>MGGSHHHHHHRSESTVTEELKEGIDAVYPSLVGTADSKAEGIKNYFKLSFTLPEEQKSRTVGSEAPLKDVAQALSSRARYELFTEKETANPAFNGEVIKRYKELMEHGEGIADILRSRLAKFLNTKDVGKRFAQGTEANRWVGGKLLNIVEQDGDTFKYNEQLLQTAVLAGLQWRLTATSNTAIKDAKDVAAITGIDQALLPEGLVEQFDTGMTLTEAVSSLAQKIESYWGLSRNPNAPLGYTKGIPTAMAAEILAAFVESTDVVENIVDMSEIDPDNKKTIGLYTITELDSFDPINSFPTAIEEAVLVNPTEKMFFGDDIPPVANTQLRNPAVRNTPEQKAALKAEQATEFYVHTPMVQFYETLGKDRILELMGAGTL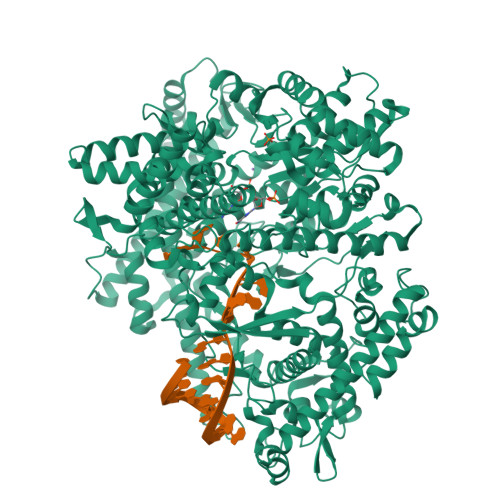NKELLNDNHAKSLEGKNRSVEDSYNQLFSVIEQVRAQSEDISTVPIHYAYNMTRVGRMQMLGKYNPQSAKLVREAILPTKATLDLSNQNNEDFSAFQLGLAQALDIKVHTMTREVMSDELTKLLEGNLKPAIDMMVEFNTTGSLPENAVDVLNTALGDRKSFVALMALMEYSRYLVAEDKSAFVTPLYVEADGVTNGPINAMMLMTGGLFTPDWIRNIAKGGLFIGSPNKTMNEHRSTADNNDLYQASTNALMESLGKLRSNYASNMPIQSQIDSLLSLMDLFLPDINLGENGALELKRGIAKNPLTITIYGSGARGIAGKLVSSVTDAIYERMSDVLKARAKDPNISAAMAMFGKQAASEAHAEELLARFLKDMETLTSTVPVKRKGVLELQSTGTGAKGKINPKTYTIKGEQLKALQENMLHFFVEPLRNGITQTVGESLVYSTEQLQKATQIQSVVLEDMFKQRVQEKLAEKAKDPTWKKGDFLTQKELNDIQASLNNLAPMIETGSQTFYIAGSENAEVANQVLATNLDDRMRVPMSIYAPAQAGVAGIPFMTIGTGDGMMMQTLSTMKGAPKNTLKIFDGMNIGLNDITDASRKANEAVYTSWQGNPIKNVYESYAKFMKNVDFSKLSPEALEAIGKSALEYDQRENATVDDIANAASLIERNLRNIALGVDIRHKVLDKVNLSIDQMAAVGAPYQNNGKIDLSNMTPEQQADELNKLFREELEARKQKVAKAR[2x]>MVEIILSHLIFDQAYFSKVWPYMDSEYFESGPAKNTFKLIKSHVNEYHSVPSINALNVALENSSFTETEYSGVKTLISKLADSPEDHSWLVKETEKYVQQRAMFNATSKIIEIQTNAELPPEKRNKKMPDVGAIPDIMRQALSISFDSYVGHDWMDDYEARWLSYMNKARKVPFKLRILNKITKGGAETGTLNVLMAGVNVGKSLGLCSLAADYLQLGHNVLYISMQMAEEVCAKRIDANMLDVSLDDIDDGHISYAEYKGKMEKWREKSTLGRLIVKQYPTGGADANTFRSLLNELKLKKNFVPTIIIVDYLGICKSCRIRVYSENSYTTVKAIAEELRALAVETETVLWTAAQVGKQAWDSSDVNMSDIAESAGLPATADFMLAVIETEELAAAEQQLIKQIKSRYGDKNKWNKFLMGVQKGNQKWVEIE[6x]

The T4 bacteriophage gp41 helicase and gp61 primase assemble into a primosome to couple DNA unwinding with RNA primer synthesis for DNA replication. The domain architecture of the gp41 helicase resembles the bacterial DnaB helicase13,14 with an NTD and a RecA-like CTD that are connected by a linking helix (LH). The gp61 primase is composed of an N-terminal ZBD and a C-terminal RPD that are linked by an 18-residue flexible loop. Here we report a series of cryo-EM structures of T4 primosome assembly intermediates.

We hypothesized that the absence of the RNA primer density in our primosome EM map was due to slow ATPγS hydrolysis by the WT gp41 helicase. Therefore, we utilized an inactive gp41 helicase mutant with an E227Q substitution in the walker-B motif that abolished the ATP-hydrolysis activity, and assembled a T4 primosome with the WT gp61 primase and the ssDNA/RNA primer substrate. We separately refined the helicase and primase regions to improve the resolution. The mutant gp41 helicase region had a resolution of 3.6 Å and revealed a structure essentially the same as the WT helicase. And the binding energy of the two additional DNA nucleotides inside the active helicase further stabilizes the active configuration. This binding-energy-driven transition hypothesis is supported by our observation that the mutant gp41 helicase, lacking ATP hydrolytic activity, also adopted the active planar ring in the assembled primosome.> ELTGFEPYDYQLRAWEKIREIMNNGGKVIIEVPTAGGKTETAVMPFFAGIYNNNWPVARLVYVLPTRSLVEKQAERLRNLVYKLLQLKGKSKEEAEKLARELVVVEYGLEKTHAFLGWVVVTTWDAFLYGLAAHRTVGNRFTFPAGAIAQSLVIFDEVQMYQDESMYMPRLLSLVVGILEEANVPLVIMSATIPSKLREMIAGDTEVITVDKNDKNKPSKGNVKVRLVEGDITDVLNDIKKILKNGKKVLVVRNTVRKAVETYQVLKKKLNDTLANPSDALLIHSRFTIGDRREKERALDSARLIVATQVVEAGLDLPNVGLVVTDIAPLDALIQRIGRCARRPGEEGEGIILIPAAAAAAAAAAAAAAAAAAAAAAAAAAAAVVTSTNEYDRVVEIHYGEGKKNFVYVGDIDTARRVLEKKRSKKLPKDLYIIPYSVSPYPDPLVLLTTYDELSKIGEYLADTTKARKALDRVYKFHYENNIVPKEFASYIYFKELKLFSAPPEYEKAAAAAAAAAAAAAAAAAAAAAAAAAAAAAAAAAAAIDAKYYNSELAAAAAAAAAAAAAAAAAAA;> FNEFKTPQIDPIFDLYVAYGYVVSLIRGGAKEATLIPHGASYLIQTDVSNEEFRHGLVDALSSMLSLHIALARHSPREGGKLVSDADFSAGANINNVYWDSVPRNLEKLMKDLEKKRSVKGTATIPITLMPSAGKYMLKHFGVQGGNPIKVDLLNYALAWVGFHYYTPYIKYAKGDTTWIHIYQIAPVEEVDMISILSLKDLKMHLPHYYESNLDFLINRRLALLYHLLHSEALELFTEKEFVIHSYTLERSGNNQAIRSFEEEEIGKLMDFLWKLKRRDFYHAIKFIDDLLKKATEGALALIDAIMNERLEGFYTALKLGKKAGVVSSREIVAALEDIIC;>GGWIRNIGRYLSYLVDDTFEEYAYDVVDGIAKARTQEELLEGVYKALRLAPKLKKKAESKGCPPPRIPSPEDIEALEEKVEQLSNPKDLRKLAVSLALWAFASWNNCP[5x];>[7x]MYVRISGRIRLNAHSLNAQGGGGTNYIEITKTKVTVRTENGWTVVEVPAITGNMLKHWHFVGFVDYFKTTPYGVNLTERALRYNGTRFGQGETTATKANGATVQLNDEATIIKELADADVHGFLAPKTGRRRVSLVKASFILPTEDFIKEVEGERLITAIKHNRVDVDEKGAIGSSKEGTAQMLFSREYATGLYGFSIVLDLGLVGIPQGLPVKFEENQPRPNIVIDPNERKARIESALKALIPMLSGYIGANLARSFPVFKVEELVAIASEGPIPALVHGFYEDYIEANRSIIKNARALGFNIEVFTYNVDLGEDIEATKVSSVEELVANLVKMV;> MDILLVCLRFPFFSVAKRSYQVRTSFLLPPPSALKGALAKGLILLKPEKYASSSLDEAALKAIKEIESKLVDIKAVSVAPLSPLIRNAFLLKRLRNLESGSNAEKSDAMRREYTFTRELLVAYIFKNLTQEEKNLYLKAAMLIDVIGDTESLATPVWASFVKPEDKKAPLAFSAPYTEIYSLLSSKIQAKGKIRMYIEKMRVSPEYSKTKGPQEEIFYLPIEERRYKRIVYYARIYPPEVEKALTVDGEVLGIWIP;> SCKAFQGQTLREHIEAMLAAWEIVKNKYIPSIIRVMKTVGVKFTEEDADKFMKTLIILHDVGKCSEVYQKHLSNNEPLRGFRHELVSAYYAYNILKDMFKDETIAFIGALVVMMHHEPILMGQIRSLDKEELTPEVVLDKLRTFNGVMEGTESFIKSMIKEKLGVIPKVPSPTQEDVLREVIRLSVLARHRPDSGKLRM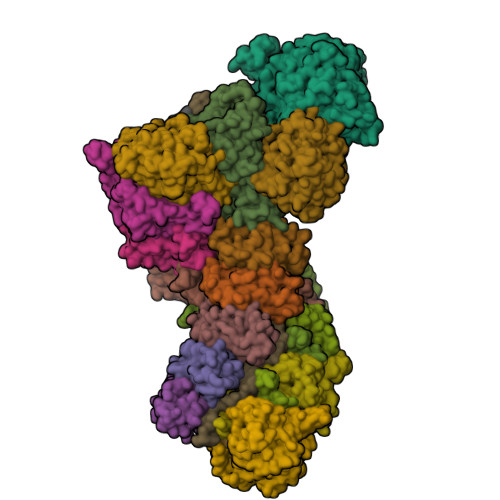VVGALLIPLVCDYKGAAAAA>MAEEHHHHHHHHLEVLFQGPGRPKTHTVGSVAKVEQVKFDATSMHVKPQVAAQQKMVDDGSGEVQVWRIENLELVPVDSKWLGHFYGGDCYLLLYTYLIGEKQHYLLYVWQGSQASQDEITASAYQAVILDQKYNGEPVQIRVPMGKEPPHLMSIFKGRMVVYQGGTSRTNNLETGPSTRLFQVQGTGANNTKAFEVPARANFLNSNDVFVLKTQSCCYLWCGKGCSGDEREMAKMVADTISRTEKQVVVEGQEPANFWMALGGKAPYANTKRLQEENLVITPRLFECSNKTGRFLATEIPDFNQDDLEEDDVFLLDVWDQVFFWIGKHANEEEKKAAATTAQEYLKTHPSGRDPETPIIVVKQGHEPPTFTGWFL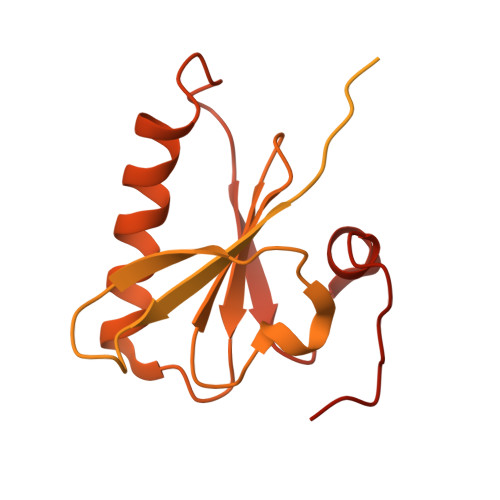AWDPFKWSGIHVVPNLSPLSNN[2x]> MSETENQALTFAKRLKADTTAVHDSVDNLVMSVQPFVSKENYIKFLKLQSVFHKAVDHIYKDAELNKAIPELEYMARYDAVTQDL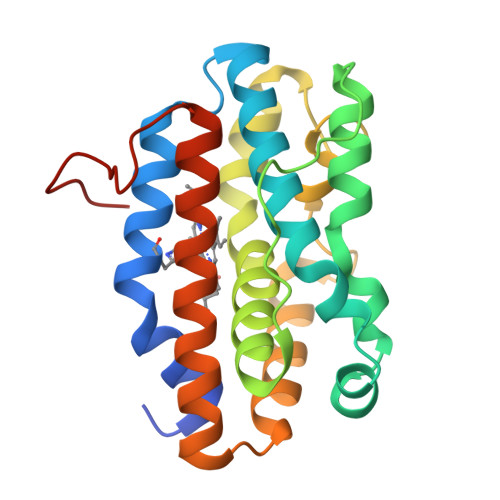KDLGEEPYKFDKELPYEAGNKAIGWLYCAEGSNLGAAFLFKHAQKLDYNGEHGARHLAPHPDGRGKHWRAFVEHLNALNLTPEAEAEAIQGAREAFAFYKVVLRETFGLAADAEAPEGMMPHRH>GPGYQMDIPKFKRLPRHIAIIPDGNRRWALARGLEKHEGYSSGIIPGLEVYDICVKIGIGEVTFFGFTQDNTKRPQIQRKAFTDACIKSVQEIAKRDAEILVVGNTNSDIFPEELLEYTKRTKVGKGKIKINFLINYGWYWDLTYAYDNSPDGKKMIENIASAEIPRVDLLIRWGGRCRLSGMLPVQTVYSDIYVVDEMWPDFKPEHLFKALEFYQNQDITLGG[8x]

MM_0014 from the methanogenic archaeon Methanosarcina mazei is known as a versatile cis-prenyltransferase that accepts both isopentenyl pyrophosphate and dimethylallyl pyrophosphate as acceptor substrates. Cis-prenyltransferase (cPT) generally catalyzes the consecutive head-to-tail condensation of isoprene units and produces (Z,E-mixed)-polyprenyl pyrophosphates. MA1831 and MM_0014, which are orthologous cPTs from the methanogenic archaea Methanosarcina acetivorans and Methanosarcina mazei, respectively, unusually accept both IPP and DMAPP as prenyl acceptor substrates. The overall structure of MM_0014 is in a ζ-fold, which is similar to those of so far reported cPTs.

With a final aim of obtaining the ternary complex structures of MM_0014 with prenyl donor and acceptor substrates, a cocrystallization of MM_0014 with FPP and Mg2+ was performed using a different crystallization buffer. The asymmetric unit of the P212121 space group contains eight protein molecules that form four homodimers. Each protein molecule possessed an electron density that penetrated the cavity more deeply than the fatty acid ligand did in the substrate-free structure. The shape of the electron density, however, did not fit well with FPP, particularly at the pyrophosphate group. It is also noteworthy that inorganic phosphate was still bound at the supposed prenyl-donor binding site and that no electron density was derived from Mg2+ ion. However, the electron density was obviously longer than farnesol (FOH), which can be produced from the hydrolysis of FPP. Thus, we speculated that the ligand was derived from the prenyltransfer reaction between FPP and glycerol because the crystallization buffer contained glycerol as a cryoprotectant. We constructed models of the possible products from the reaction, i.e., 1-O-farnesyl-sn-glycerol (FG), 2-O-FG, and 3-O-FG, and fitted them with the electron density. A 1:1:1 mixture of the models seemed to fit better than each model, suggesting that different O-prenylation products are formed and bound in MM_0014.> MHLNPAEKEKLQIFLASELALKRKARGLKLNYPEAVAIITSFIMEGARDGKTVAMLMEEGKHVLTRDDVMEGVPEMIDDIQAEATFPDGTKLVTVHNPIS;> NYIVPGEYRVAEGEIEINAGREKTTIRVSNTGDRPIQVGSHIHFVEVNKELLFDRAEGIGRRLNIPSGTAARFEPGEEMEVELTELGGNREVFGISDLTNGSVDNKELILQRAKELGYKGVE;> MKINRQQYAESYGPTVGDQVRLADTDLWIEVEKDYTTYGDEANFGGGKVLREGMGENGTYTRTENVLDLLLTNALILDYTGIYKADIGVKDGYIVGIGKGGNPDIMDGVTPNMIVGTATEVIAAEGKIVTAGGIDTHVHFINPDQVDVALANGITTLFGGGTGPAEGSKATTVTPGPWNIEKMLKSTEGLPINVGILGKGHGSSIAPIMEQIDAGAAGLKIHEDWGATPASIDRSLTVADEADVQVAIHSDTLNEAGFLEDTLRAINGRVIHSFHVEGAGGGHAPDIMAMAGHPNVLPSSTNPTRPFTVNTIDEHLDMLMVCHHLKQNIPEDVAFADSRIRPETIAAEDILHDLGIISMMSTDALAMGRAGEMVLRTWQTADKMKKQRGPLAEEKNGSDNFRAKRYVSKYTINPAIAQGIAHEVGSIEEGKFADLVLWEPKFFGVKADRVIKGGIIAYAQIGDPSASIPTPQPVMGRRMYGTVGDLIHDTNITFMSKSSIQQGVPAKLGLKRRIGTVKNCRNIGKKDMKWNDVTTDIDINPETYEVKVDGEVLTCEPVKELPMAQRYFLF

Urease, depending on the organism, is a nickel-containing homo- or heterooligomeric amidohydrolase that is commonly expressed in plants, fungi, and bacteria, but not in animals/humans, and catalyzes the decomposition of urea to ammonia and carbonate. The activity of urease in microorganisms, which in turn determines the accumulation of NH3 and the increase in pH in the microbial microenvironment, is a key factor contributing to the persistence of notorious bacterial infections. Organoselenium compounds, and, in particular, Ebselen, have been classified among the most potent low-molecular-weight inhibitors of bacterial ureases. Although Ebselen is considered to act as a broad-band thiol-targeted inhibitor, it inactivated S. pasteurii urease (SPU) with a Ki of 2.11 nM, an exceptional value among mammalian or bacterial enzymes.

Crystallographic studies on SPU inhibited by the most efficient Ebselen derivative reveal the molecular basis for this striking reactivity, namely, the formation of a unique chemical modification of the catalytic cysteine thiol, a novel mechanism of urease inhibition. The Ni-containing active site region is completely conserved with respect to that of the native S. pasteurii urease, with the dinuclear Ni(1)–Ni(2) cluster (where the two Ni ions are 3.7 Å far apart) being bridged by the Oθ1 and Oθ2 atoms of a carbamoylated αLys220* residue and a hydroxide ion W(B). The unbiased omit electron density Fourier map calculated before the addition of the ligands in the refined model revealed two positive and unmodeled regions in proximity of the two solvent-exposed cysteine residues of SPU, namely, αCys322 and αCys555, thus suggesting covalent adducts formed on the Sγ atoms of those residues. The unmodeled electron density peak located next to αCys322* revealed a peculiar oblong shape, suggesting the presence of two spherical ligands possibly forming a dinuclear Se cluster bound to the Sγ atom of αCys322*. Similarly, the anomalous difference electron density Fourier map showed an oblong shape overlapping to the omit map, confirming the attribution of two Se atoms, which were therefore both successfully modeled and refined with a 70% occupancy: Se(1) was refined bound to αCys322* Sγ at ca. 2.2 Å, while Se(2) was refined bound to Se(1) at ca. 2.3 Å. The electron density proximal to αCys555* revealed a different kind of binding. The electron density was successfully interpreted by modeling 47 with full occupancy and bound to the αCys555* Sγ atom through its Se atom (at ca. 2.4 Å). The mobile flap region of the determined X-ray crystal structure of SPU bound to two Se atoms was found in the open state, with a mainly conserved protein backbone conformation with respect to that of the native enzyme.> EVWTQRLHGGSAPLPQDRGFLVVQGDPRELRLWARGDARGASRADEKPLRRKRSAALQPEPIKVYGQVSLNDSHNQMVVHWAGEKSNVIVALARDSLALARPKSSDVYVSYDYGKSFKKISDKLNFGLGNRSEAVIAQFYHSPADNKRYIFADAYAQYLWITFDFCNTLQGFSIPFRAADLLLHSKASNLLLGFDRSHPNKQLWKSDDFGQTWIMIQEHVKSFSWGIDPYDKPNTIYIERHEPSGYSTVFRSTDFFQSRENQEVILEEVRDFQLRDKYMFATKVVHLLGSEQQSSVQLWVSFGRKPMRAAQFVTRHPINEYYIADASEDQVFVCVSHSNNRTNLYISEAEGLKFSLSLENVLYYSPGGAGSDTLVRYFANEPFADFHRVEGLQGVYIATLINGSMNEENMRSVITFDKGGTWEFLQAPAFTG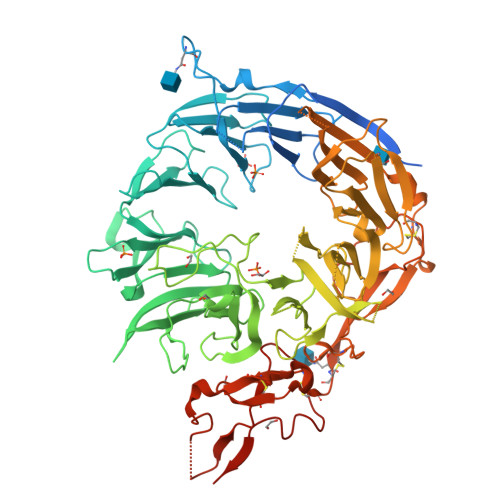YGEKINCELSQGCSLHLAQRLSQLLNLQLRRMPILSKESAPGLIIATGSVGKNLASKTNVYISSSAGARWREALPGPHYYTWGDHGGIITAIAQGMETNELKYSTNEGETWKTFIFSEKPVFVYGLLTEPGEKSTVFTIFGSNKENVHSWLILQVNATDALGVPCTENDYKLWSPSDERGNECLLGHKTVFKRRTPHATCFNGEDFDRPVVVSNCSCTREDYECDFGFKMSEDLSLEVCVPDPEFSGKSYSPPVPCPVGSTYRRTRGYRKISGDTCSGGDVEARLEGELVPCPSRLENLYFQ>SNAMSPIIAPPAELVDPKDRVQLRRVFGDFPTGVTVVTVGGSEPRGMTANSFTSVSLSPPLVLICVGKDAVMHQRLTALPTFAVSVLE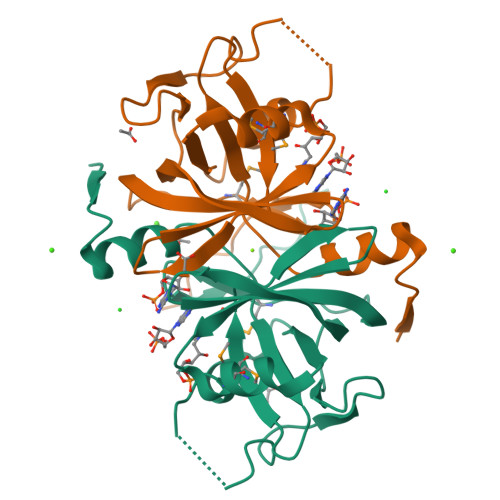AGQEKAARHFADHSRPPGVDQFDTVDWVLGEESGAPLIAGAVAHLECAIHRLYEGGDHTIFLGEVITATRWPAREGMLFSGGRFRRFAPDADEGRAA[2x]> MNAACAVDAGSVDQTVQLGQVRTASLAQEGATSSAVGFNIQLNDCDTN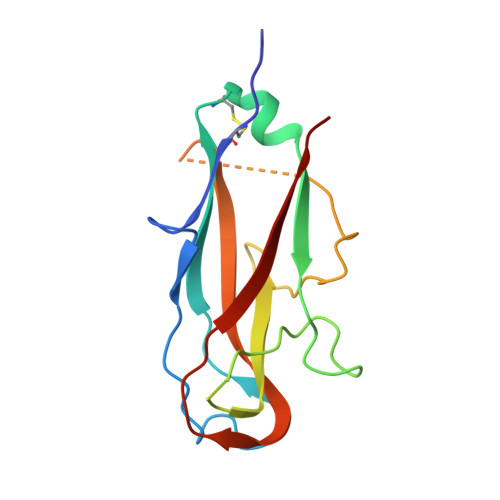VASKAAVAFLGTAIDAGHTNVLALQSSAAGSATNVGVQILDRTGAALTLDGATFSSETTLNNGTNTIPFQARYFATGAATPGAANADATFKVQYQ> MSKPQPIAAANWKSGSPDSLSELIDLFNSTSIN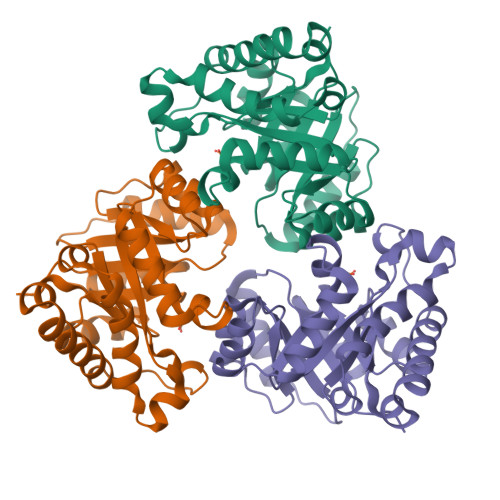HDVQCVVASTFVHLAMTKERLSHPKFVIAAQNAGNADALASLKDFGVNWIVLGHSERRWYYGETNEIVADKVAAAVASGFMVIACIGETLQERESGRTAVVVLTQIAAIAKKLKKADWAKVVIAYEPVWAIGTGKVLTPQQAQEAHALIRSWVSSKIGADVAGELRILYGGSVNGKNARTLYQQRDVNGFLVGGASLKPEFVDIIKATQ> SSLDDKPQFPGASAEFIDKLEFIQPNVISGIPIYRVMDRQGQIINPSEDPHLPKEKVLKLYKSMTLLNTMDRILYESQRQG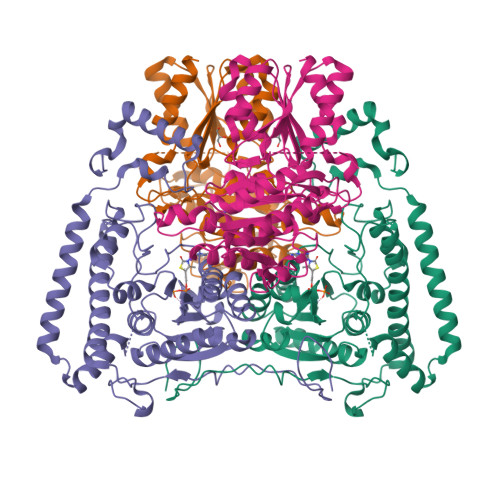RISFYMTNYGEEGTHVGSAAALDNTDLVFGQFREAGVLMYRDYPLELFMAQCYGNISDLGKGRQMPVHYGCKERHFVTISSPLATQIPQAVGAAYAAKRANANRVVICYFGEGAASEGDAHAGFNFAATLECPIIFFCRNNGYAISTPTSEQYRGDGIAARGPGYGIMSIRVDGNDVFAVYNATKEARRRAVAENQPFLIEAMTYRIGHASTSDDSSAFRSVDEVNYWDKQDHPISRLRHYLLSQGWWDEEQEKAWRKQSRRKVMEAFEQAERKPKPNPNLLFSDVYQEMPAQLRKQQESLARHLQTYGEHYPLDHFDK;> VAHFTFQPDPEPREYGQTQKMNLFQSVTSALDNSLAKDPTAVIFGEDVAFGGVFRCTVGLRDKYGKDRVFNTPLCEQGIVGFGIGIAVTGATAIAEIQFADYIFPAFDQIVNEAAKYRYRSGDLFNCGSLTIRSPWGCVGHGALYHSQSPEAFFAHCPGIKVVIPRSPFQAKGLLLSCIEDKNPCIFFEPKILYRAAAEEVPIEPYNIPLSQAEVIQEGSDVTLVAWGTQVHVIREVASMAKEKLGVSCEVIDLRTIIPWDVDTICKSVIKTGRLLISHEAPLTGGFASEISSTVQEECFLNLEAPISRVCGYDTPFPHIFEPFYIPDKWKCYDALRKMINY6-aminopyrimidine-2,4(3H,5H)-dione | C4 H5 N3 O2 | 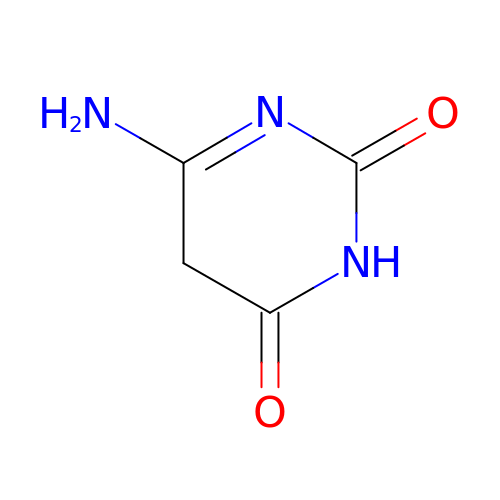BLOCGUWRFAOSFW-UHFFFAOYSA-N>[2x]DTYQKEIEDKKIS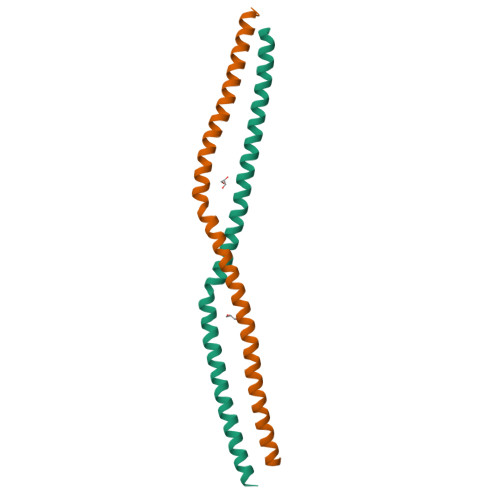EENLLEEVEKAKVIADEAVKLQKEIDKRCQHKIAEMVALMEKHKHQYDKIIEERDSELGLYKSKEQEQSSLRASLEIELSNLKAELLSVKKQLEIEREEKEKLKREAKENTATLKEKKDKKTQTFLLLEHHHHHH> GAMGIRNSMGQEPRTLPPSPNWYCARCSDAVPGGLFGFAARTSVFLVRVGPGAGESPGTPPFRVIGELVGHTERVSGFTFSHHPGQYNLCATSSDDGTVKIWDVETKTVVTEHALHQHTISTLHWSPRVKDLIVSGDEKGVVFCYWFNRNDSQHLFIEPRTIFCLTCSPHHEDLVAIGYKDGIVVIIDISKKGEVIHRLRGHDDEIHSIAWCPLPGEDCLSINQEETSEEAEITNGNAVAQAPVTKGCYLATGSKDQTIRIWSCSRGRGVMILKLPFLKRRGGGIDPTVKERLWLTLHWPSNQPTQLVSSCFGGELLQWDLTQSWRRKYTLFSASSEGQNHSRIVFNLCPLQTEDDKQLLLSTSMDRDVKCWDIATLECSWTLPSLGGFAYSLAFSSVDIGSLAIGVGDGMIRVWNTLSIKNNYDVKNFWQGVKSKVTALCWHPTKEGCLAFGTDDGKVGLYDTYSNKPPQISSTYHKKTVYTLAWGPPVPPMSLGGEGDRPSLALYSCGGEGIVLQHNPWKLSGEAFDINKLIRDTNSIKYKLPVHTEISWKADGKIMALGNEDGSIEIFQIPNLKLICTIQQHHKLVNTISWHHEHGSQPELSYLMASGSNNAVIYVHNLKTVIESSPESPVTITEPYRTLSGHTAKIT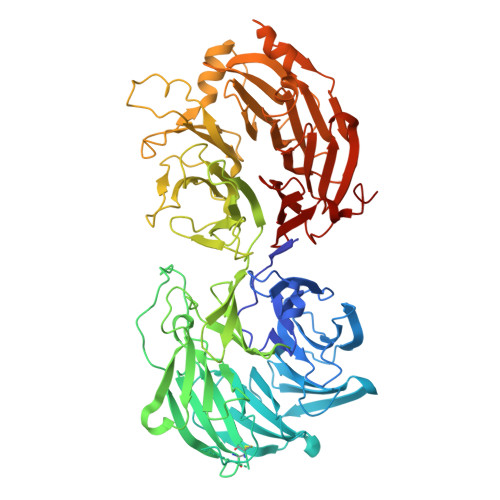SVAWSPHHDGRLVSASYDGTAQVWDALREEPLCNFRGHRGRLLCVAWSPLDPDCIYSGADDFCVHKWLTSMQDHSRPPQGKKS> MLTMKDIIRDGHPTLRQKAAELELPLTKEEKETLIAMREFLVNSQDEEIAKRYGLRSGVGLAAPQINISKRMIAVLIPDDGSGKSYDYMLVNPKIVSHSVQEAYLPTGEGCLSVDDNVAGLVHRHNRITIKAKDIEGNDIQLRLKGYPAIVFQHEIDHLNGVMFY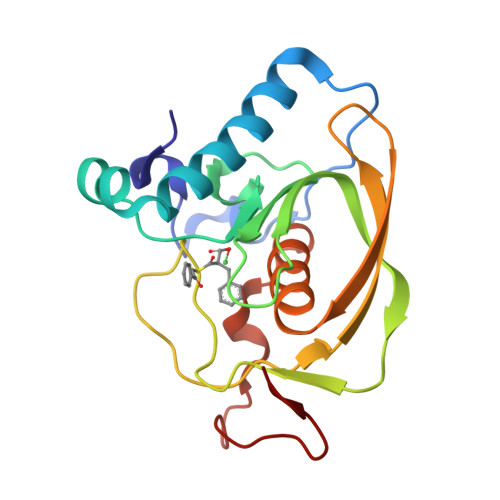DHIDKNHPLQPHTDAVEV>GSHMASNKYKRIFLVVMDSVGIGEAPDAEQFGDLGSDTIGHIAEHMNGLQMPNMVKLGLGNIREMKGISKVEKPLGYYTKMQEKSTGKDQMTGHWEIMGLYIDTPFQVFPEGFPKELLDELEEKTGRKIIGNKPASGTEILDELGQEQMETGSLIVYTSADSVLQIAAHEEVVPLDELYKICKIARELTLDEKYMVGRVIARPFVGEPGNFTRTPNRHDYALKPFGRTVMNELKDSDYDVIAIGKISDIYDGEGVTESLRTKSNMDGMDKLVDTLNMDFTGLSFLNLVDFDALFGHRRDP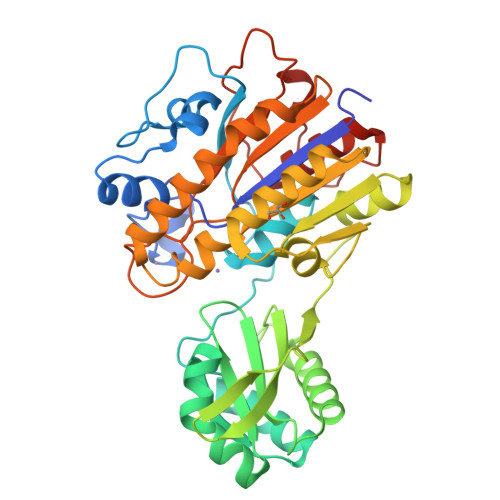QGYGEALQEYDARLPEVFAKLKEDDLLLITADHGNDPIHPGTDHTREYVPLLAYSPSMKEGGQELPLRQTFADIGATVAENFGVKMPEYGTSFLNELKK[3x]> ALVKEEIQAKEYLENLNKELAKRTNVETEAAWAYGSNITDENEKKKNEISAELAKFMKEVASDTTKFQWRSYQSEDLKRQFKALTKLGYAALPEDDYAELLDTLSAMESNFAKVKVCDYKDSTKCDLALDPEIEEVISKSRDHEELAYYWREFYDKAGTAVRSQFERYVELNTKAAKLNNFTSGAEAWLDEYEDDTFEQQLEDIFADIRPLYQQIHGYVRFRLRKHYGDAVVSETGPIPMHLLGNMWAQQWSEIADIVSPFPEKPLVDVSAEMEKQGYTPLKMFQMGDDFFTSMNLTKLPQDFWDKSIIEKPTDGRDLVCHASAWDFYLTDDVRIKQCTRVTQDQLFTVHHELGHIQYFLQYQHQPFVYRTGANPGFHEAVGDVLSLSVSTPKHLEKIGLLKDYVRDDEARINQLFLTALDKIVFLPFAFTMDKYRWSLFRGEVDKANWNCAFWKLRDEYSGIEPPVVRSEKDFDAPAKYHISADVEYLRYLVSFIIQFQFYKSACIKAGQYDPDNVELPLDNCDIYGSAAAGAAFHNMLSMGASKPWPDALEAFNGERIMSGKAIAEYFEPLRVWLEAENIKNNVHIGWTTSNKCVS;> EGLPPRPKIPP

Peptidyl dipeptidase A is a highly glycosylated ectoenzyme that cleaves dipeptides from the C-terminus of a broad range of oligopeptides. AnCE is a single-domain glycosylated protein that closely shares enzymatic properties with human ACE (in particular the C-domain of human somatic ACE) and is inhibited by classic inhibitors of the human enzymes 14–17. In this study, we elucidate how the natural peptides Ang II (the principal end-product of the renin-angiotensin–aldosterone system), Arg–Pro–Pro (the BK-derived peptide) and bradykinin-potentiating peptide-b (BPPb, a snake venom inhibitor) bind to the active site of AnCE, revealing novel interactions involving several enzyme subsites. Comparison of the four structures clearly shows a common mode of peptide binding to AnCE.

BPPb is one of several blood-pressure-lowering peptides isolated from the venom of Bothrops jararaca and has been shown to be an inhibitor of D. melanogaster AnCE and both domains of human somatic ACE, but with > 200-fold selectivity towards the C-domain. For the inhibitory BPPb peptide (pGlu–Gly–Leu–Pro–Pro–Arg–Pro–Lys–Ile–Pro–Pro; Ki, 107 μm) clear continuous electron density was observed for residues Arg–Pro–Lys–Ile–Pro–Pro. The structure of the AnCE–BPPb complex revealed interactions between the pyrrolidine ring of the two Pro residues in the penultimate and C-terminal positions (P1′ and P2′, respectively) and the amino acid side chains that form the S1′ and S2′ enzyme subsites, respectively. A cluster of aromatic residues forms this binding pocket (Phe441, Phe511, Tyr504, Tyr507), and Tyr507 ‘stacks’ against the C-terminal Pro, thus enhancing the interaction with AnCE. The two Pro residues (P1′ and P2′) are strongly anchored in the prime binding sites (S1′ and S2′) by hydrogen bonding with multiple residues. The P2′ Pro, in particular, has strong interactions with Gln265, Tyr504 and Lys495. The Ile residue from the BPPb peptide forms a direct coordination with the catalytic zinc ion by replacing the usual water molecule observed in the native AnCE structure 18. This residue is further stabilized by interaction with the hydroxyl group of Tyr507. The main chain of the next Lys residue of the peptide in the P2 position interacts with Ala340 through two hydrogen bonds. Of the two visible N-terminal residues of BPPb, namely Pro and Arg, Pro is stabilized by hydrophobic interaction with a bulky Trp341 residue, whereas the Arg side chain forms a weak interaction with AnCE via a water-mediated hydrogen bond with Asp501.>GSSMDNQDGFILQQVKLSLDDPDSYLSSWNSNDASPCRWSGVSCAGDFSSVTSVDLSSANLAGPFPSVICRLSNLAHLSLYNNSINSTLPLNIAACKSLQTLDLSQNLLTGELPQTLADIPTLVHLDLTGNNFSGDIPASFGKFENLEVLSLVYNLLDGTIPPFLGNISTLKMLNLSYNPFSPSRIPPEFGNLTNLEVMWLTECHLVGQIPDSLGQLSKLVDLDLALNDLVGHIPPSLGGLTNVVQIELYNNSLTGEIPPELGNLKSLRLLDASMNQLTGKIPDELCRVPLESLNLYENNLEGELPASIALSPNLYEIRIFGNRLTGGLPKDLGLNSPLRWLDVSENEFSGDLPADLCAKGELEELLIIHNSFSGVIPESLADCRSLTRIRLAYNRFSGSVPTGFWGLPHVNLLELVNNSFSGEISKSIGGASNLSLLILSNNEFTGSLPEEIGSLDNLNQLSASGNKFSGSLPDSLMSLGELGTLDLHGNQFSGELTSGIKSWKKLNELNLADNEFTGKIPDEIGSLSVLNYLDLSGNMFSGKIPVSLQSLKLNQLNLSYNRLSGDLPPSLAKDMYKNSFIGNPGLCGDIKGLCGSENEAKKRGYVLEGSENLYFQ[2x];>[2x]GSSMASANLEGDALHTLRVTLVDPNNVLQSWDPTLVNPCTWFHVTCNNENSVIRVDLGNAELSGHLVPELGVLKNLQYLELYSNNITGPIPSNLGNLTNLVSLDLYLNSFSGPIPESLGKLSKLRFLRLNNNSLTGSIPMSLTNITTLQVLDLSNNRLSGSVPDNGSFSLFTPISFANNLDLCGPVTSHPCPGSLENLYFQ;>PVPTSGPSRKHN[2x]

Here we demonstrate that HSL1 binds IDA/IDL peptides with high, and CLE peptides with lower affinity, respectively. Ligand sensing capability and receptor activation of HSL1 require a SERK co-receptor kinase. Crystal structures with IDA/IDLs or with CLE9 reveal that HSL1-SERK1 complex recognizes the entire IDA/IDL signaling peptide, while only parts of CLE9 are bound to the receptor. Our work reveals that HSL1 is a receptor for IDA/IDL signaling peptides.

The vastly different binding affinities between IDA/IDLs vs. CLE9 to HSL1 prompted us to determine co-crystal structures of four HSL1-IDA/IDL-SERK1 ternary complexes with: IDA, IDL1, IDL2, and IDL3 (at 2.31 Å, 2.38 Å, 2.20 Å, and 2.70 Å, respectively) and the HSL1-CLE9-SERK1 complex at 2.87 Å. In agreement with our biochemical assays, the crystal structures revealed that all IDA/IDL peptides specifically bind to the peptide-binding surface of HSL1. IDA/IDLs adopt a fully extended conformation in the structure. The co-receptor SERK1 interacts with the C-terminal region of the different IDA/IDL peptides (residues 68-69 in IDA), completing the peptide-binding pocket using its N-terminal loop region. Superposition of the four crystal structures yielded an R.M.S.D of ~0.6 Å comparing 590 Cα atom pairs, with IDL peptides perfectly aligning to each other. HSL1 forms stable heterodimeric complexes with SERK1 in the presence of IDA/IDL peptides in analytical size-exclusion chromatography experiments (SEC). However, HSL1 displays an extended hydrogen-bonding network in its core ligand interaction surface, accounting for the higher binding affinity to IDA/IDL peptides when compared to HAESA.>[2x]MGSGLKAGDSFPSDVVFSYIPWSEDKGEITASGIPINYNASKEWADKKVILFALPGAFTPVSSARH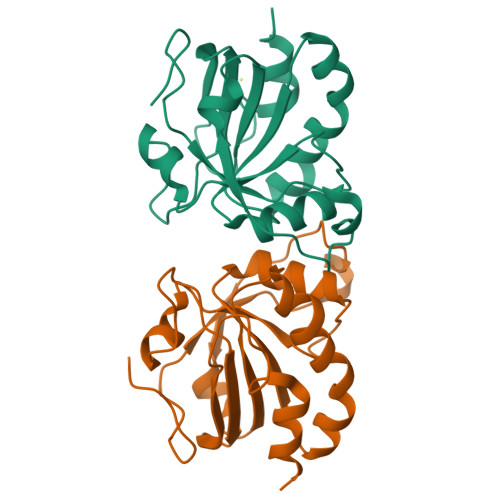VPEYIEKLPEIRAKGVDVVAVLAYNDAYVMSAWGKANQVTGDDILFLSDPDARFSKSIGWADEEGRTKRYALVIDHGKITYAALEPAKNHLEFSSAETVLKHLHHHHHH>GGGAGCCCU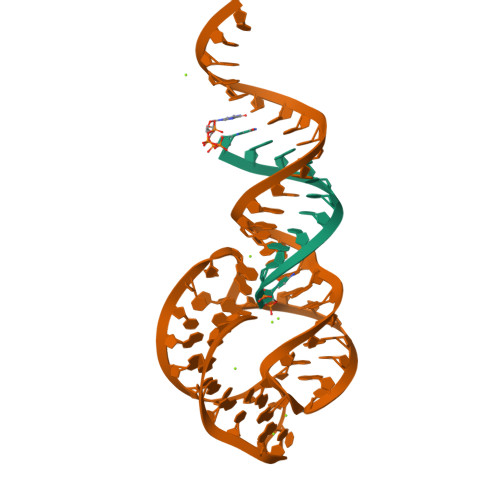GUC[2x];>[2x]ACCGGAUGUGCUUUCCGGUCUGAUGAGUCCGUGAGGACAAAACAGGGCUCCCGAAUU> GAMGAKVVIEPHRHAGVYIARGKEDLLVTKNMAPGESVYGEKRISVEEPSKEDGVPPTKVEYRVWNPFRSKLAAGIMGGLDELFIAPGKKVLYLGAASGTSVSHVSDVVGPEGVVYAVEFSHRPGRELISMAKKRPNIIPIIEDARHPQKYRMLIGMVDCVF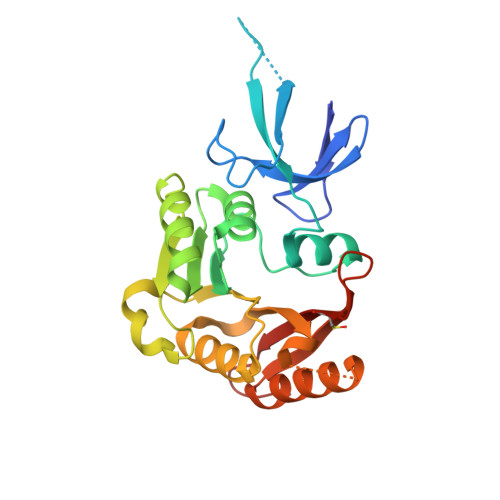ADVAQPDQARIIALNSHMFLKDQGGVVISIKANCIDSTVDAETVFAREVQKLREERIKPLEQLTLEPYERDHCIVVGRYMRSGLKK> AMKKDSKAP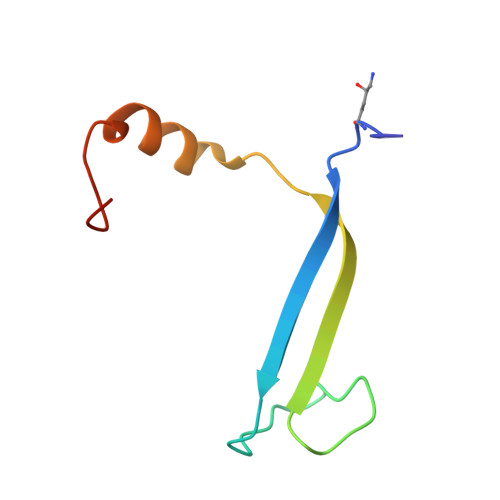CVEVFDERDGCKAAGTQKASGDDGFCVKVSMKAIGFNAAEAASVTKNYGIKRFGAKSV> GSMREYKLVVLGSVGVGKSALTVQ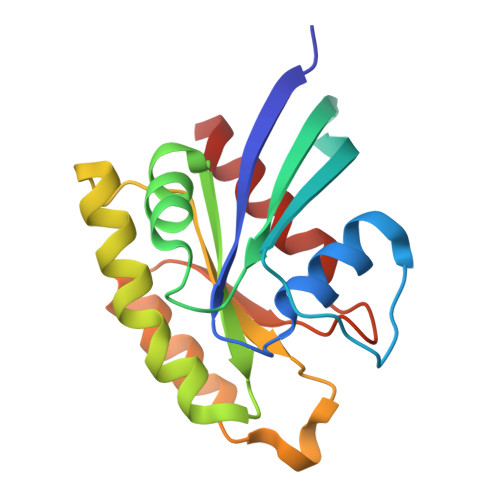FVQGIFVEKYDPTIEDSYRKQVEVDAQQCMLEILDTAGTEQFTAMRDLYMKNGQGFALVYSITAQSTFNDLQDLREQILRVKDTDDVPMILVGNKCDLEDERVVGKEQGQNLARQWNNCAFLESSAKSKINVNEIFYDLVRQINR> DQAGKSPNAVRYHGGDEIILQGFHWNVVREAPNDWYNILRQQAATIAADGFSAIWMPVPWRDFSSWSDGSKSGGGEGYFWHDFNKNGRYGSDAQLRQAASALGGAGVKVLYDVVPNHMNRGYPDKEINLPAGQGFWRNDCADPGNYPNDCDDGDRFIGGDADLNTGHPQVYGMFRDEFTNLRSQYGAGGFRFDFVRGYAPERV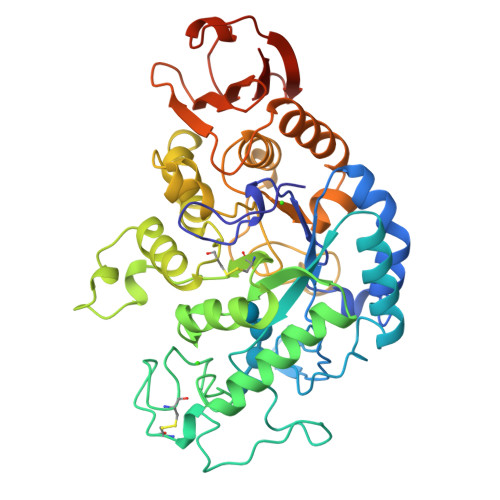NSWMTDSADNSFCVGGLWKGPSEYPNWDWRNTASWQQIIKDWSDRAKCPVFDFALKERMQNGSIADWKHGLNGNPDPRWREVAVTFVDNHDTGYSPGQNGGQHHWALQDGLIRQAYAYILTSPGTPVVYWDHMYDWGYGDFIRQLIQVRRAAGVRADSAISFHSGYSGLVATVSGSQQTLVVALNSDLGNPGQVASGSFSEAVNASNGQVRVWRSGTGSGGGEPGA>[4x]MEELQDDYEDMMEENLEQEEYEDPDIPESQMEEPAAHDTEATATDYHTTSHPGTHKVYVELQELVMDEKNQELRWMEAARWVQLEENLGENGAWGRPHLSHLTFWSLLELRRVFTKGTVLLDLQETSLAGVANQLLDRFIFEDQIRPQDREELLRALLLKHSHAGELEALGGVKPAVLTRSGDPSQPLLPQHSSLETQLFCEQGDGGTEGHSPSGILEKIPPDSEATLVLVGRADFLEQPV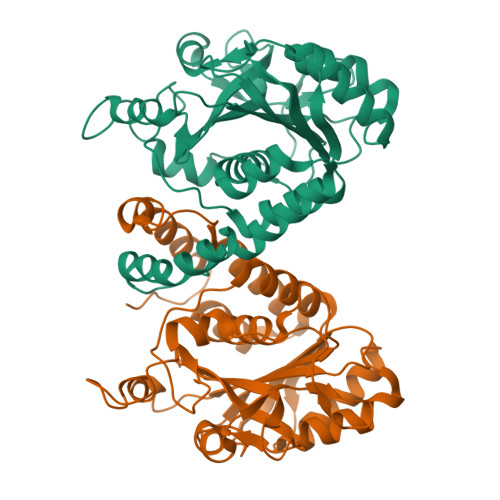LGFVRLQEAAELEAVELPVPIRFLFVLLGPEAPHIDYTQLGRAAATLMSERVFRIDAYMAQSRGELLHSLEGFLDCSLVLPPTDAPSEQALLSLVPVQRELLRRRYQSSPAKPDSSFYKGLDLNGGPDDPLQQTGQLF>SNAMSTDRESQLLRQATKAGIDSPLELANFMAQAGHESRGLSRLNESFNFTRGISQIPVEAAWRNGNAALESARQEALRGRPENLAELMYGGRMGNDAPGDALKYHGRGYLPLVGKENYERAGKALDLDLVNQPELAAQPEHAGRIAVWQWQTRVPEGARHDVREATYALNGALNGIEARRQRFEVWQQKLTPDVMARLDRGEVGAPAQTVARDMSHAGEPGNALFEDARQHLRQMGPQSGLRSAQELDNTAGALALGAQKAGLSRIDHLLAGNDGRTLFAVQGALGDPAMLRASVDREQASQQSLAQSSQQLAASVAQQDPTAALAREQEQRSRSL[2x]

Stenotrophomonas maltophilia expresses a type IV protein secretion system (T4SS) that promotes contact-dependent killing of other bacteria and does so partly by secreting the effector TfcB. Here, we report the structure of TfcB, comprising an N-terminal domain similar to the catalytic domain of glycosyl hydrolase (GH-19) chitinases and a C-terminal domain for recognition and translocation by the T4SS. Thus, TfcB is comprised of a fold similar to that of characterized GH-19 chitinases/endolysin. Furthermore, the SPN1S protein’s apical head-like domain is important for interactions with peptidoglycan. These analyses demonstrate that TfcB shares significant structural homology with GH-19 enzymes and may target a component of bacterial cell walls.

As a result, we determined the structure of TfcB to 1.9 Å. There are two molecules of TfcB in the asymmetric unit. Each protomer consists of 12 α helices, 2–310 helices, and 3 β sheets and forms two domains. The N-terminal domain is composed of two helical bundles. Helical bundle A (η1–η2, α3–α6) forms an apical head-like region that is linked to bundle B (α1, α2, α8, and α9) by long helix α7 and loop 2 (L2 connects α2 and η1). These helical bundles connect to create a cleft or concave groove that consists primarily of residues from L2 and loop 3 (L3) that connects α5 and α6 and protrudes down into this groove. The C-terminal domain is composed of a single helical bundle (α10, α11, and α12) adjacent to a three-stranded, anti-parallel β-sheet. Structural overlay of TfcB to that of these GH-19 enzymes showed that residues Glu34 and Glu43 of TfcB align with the catalytic Glu residues of the well-characterized chitinases. However, Val111 aligns with the Ser/Thr residue of the conserved GH-19 catalytic triad. The Ser-to-Val substitution in the catalytic triad of TfcB and numerous non-conserved amino-acid substitutions in the substrate binding motif suggested that this effector possibly targets a substrate other than GlcNAc or chitin.> GVPTYLLPGSSQFMTTDDHSSAPAFPDFSPTPEIHIPGRVHNMLELVQVESMMEINNVAGSSGMERLRVEISVQTDMDALLFNIPLDIQLDGPLRSTLLANIARYYTHWSGSMEMTFMFCGSFMATGKVILCYTPPGGSCPTDRESA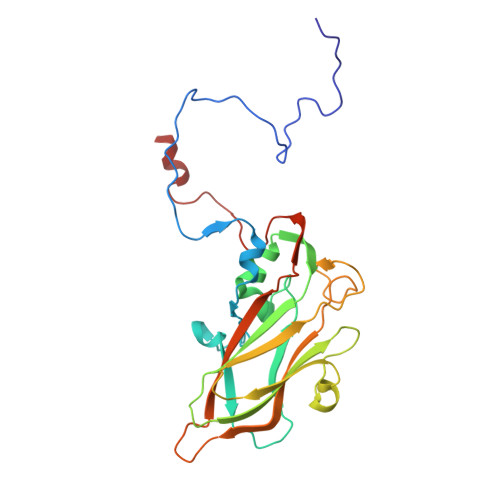MLGTHIVWDFGLQSSITLVIPWISGSHFRMFNSDAKSINANVGYVTCFMQTNLIVPKEAATSTYIIGFAAAKNDFSLRLMRDSPDIGQSQQLEGATAAFQ>[8x]MSELKTGHAGHNPWASVANSGPISILSYCGSSILMTVTNKFVVNLKDFNMNFVMLFVQSLVCTITLIILRILGYAKFRSLNKTDAKNWFPISFLLVLMIYTSSKALQY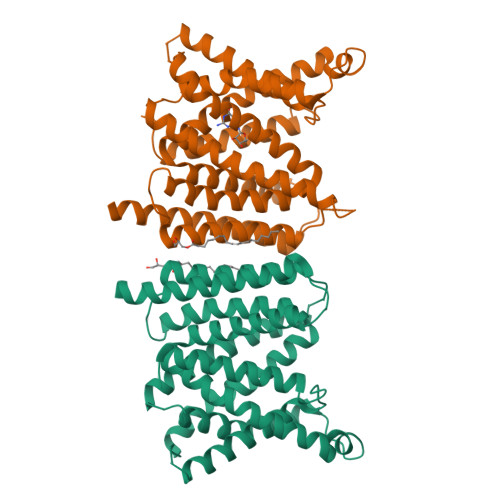LAVPIYTIFKNLTIILIAYGEVLFFGGSVTSMELSSFLLMVLSSVVATWGDQQAVAAKAASLAEGAAGAVASFNPGYFWMFTNCITSALFVLIMRKRIKLTNFKDFDTMFYNNVLALPILLLFSFCVEDWSSVNLTNNFSNDSLTAMIISGVASVGISYCSGWCVRVTSSTTYSMVGALNKLPIALSGLIFFDAPRNFLSILSIFIGFLSGIIYAVAKQKKQQAQPLRK> NTIELFYMPSDEELTANPNALQEASFTEEDINGLKGVDGVKQVVASAVKSMTARYHEEDT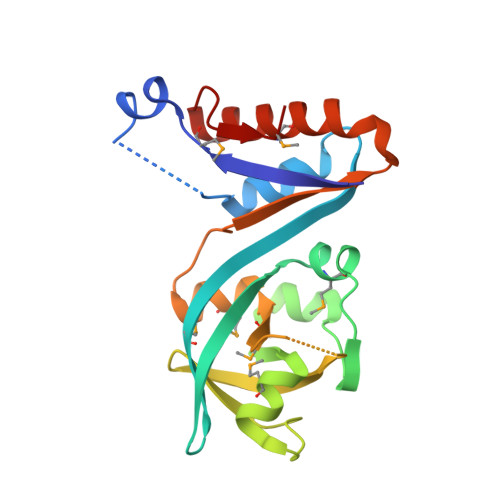DITLNGINSGYMDVKKLDVQDGRTFTDNDFLSGKRAGIISKKMAEKLFGKTSPLGKIVWAGGQPVEVIGVLKEESGFLSLGLSEMYVPFNMLKTSFGTNDYSNVSVQTESADQIKSTGKEAARLLNDNHGTKEAYQVMN> NTMKYIKAADFQSAFKAVNREILENPQFVTDSRIGRCNEIGSMTVVVDTPSSFKMTDPRINRIS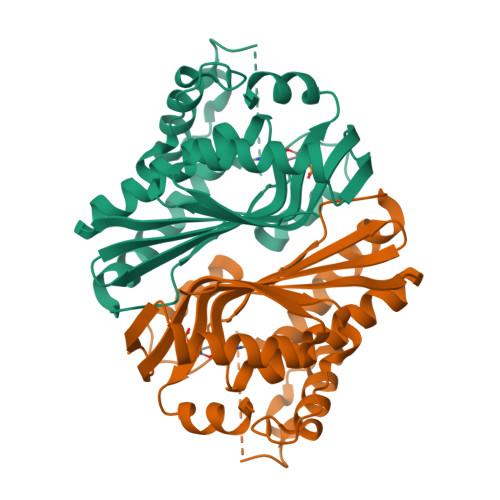YEYAEDFWKFMISGGTDAKEAFKAYPNVAKFISKPKSDALPANFNTFYGPRIAAQLPALLKELKEKPNSRRVVFQILESSDQALLDSDETLEYPCTDSVTYYIRDGKLYTHCHMRSQNCAVVMQLDFYLQGKLLHYIANECGVEVGDYTHTMVSAHVFERDFDYVKGFLD>AQAGHYITKNGNDWQYDTNGELAKGLRQDSNGKLRYFDLTTGIQAKGQFVTIGQETYYFSKDHGDAQLLPMVTEGHYGTITLKQGQDTKTAWVYRDQNNTILKGLQNINGTLQFFDPYTGEQLKGGVAKY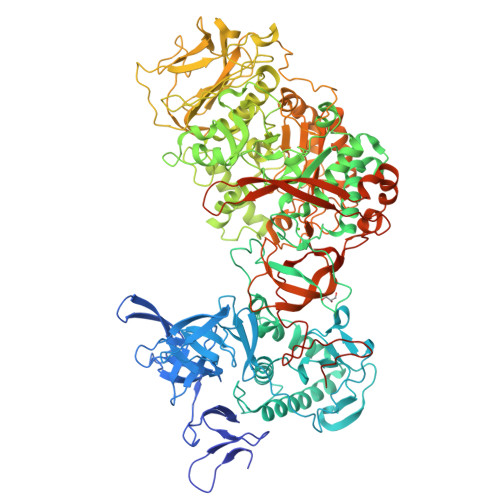DDKLFYFESGKGNLVSTVAGDYQDGHYISQDGQTRYADKQNQLVKGLVTVNGALQYFDNATGNQIKNQQVIVDGKTYYFDDKGNGEYLFTNTLDMSTNAFSTKNVAFNHDSSSFDHTVDGFLTADTWYRPKSILANGTTWRDSTDKDMRPLITVWWPNKNVQVNYLNFMKANGLLTTAAQYTLHSDQYDLNQAAQDVQVAIERRIASEHGTDWLQKLLFESQNNNPSFVKQQFIWNKDSEYHGGGDAWFQGGYLKYGNNPLTPTTNSDYRQPGNAFDFLLANDVDNSNPVVQAENLNWLHYLMNFGTITAGQDDANFDSIRIDAVDFIHNDTIQRTYDYLRDAYQVQQSEAKANQHISLVEAGLDAGTSTIHNDALIESNLREAATLSLTNEPGKNKPLTNMLQDVDGGTLITDHTQNSTENQATPNYSIIHAHDKGVQEKVGAAITDATGADWTNFTDEQLKAGLELFYKDQRATNKKYNSYNIPSIYALMLTNKDTVPRMYYGDMYQDDGQYMANKSIYYDALVSLMTARKSYVSGGQTMSVDNHGLLKSVRFGKDAMTANDLGTSATRTEGLGVIIGNDPKLQLNDSDKVTLDMGAAHKNQKYRAVILTTRDGLATFNSDQAPTAWTNDQGTLTFSNQEINGQDNTQIRGVANPQVSGYLAVWVPVGASDNQDARTAATTTENHDGKVLHSNAALDSNLIYEGFSNFQPKATTHDELTNVVIAKNADVFNNWGITSFEMAPQYRSSGDHTFLDSTIDNGYAFTDRYDLGFNTPTKYGTDGDLRATIQALHHANMQVMADVVDNQVYNLPGKEVVSATRAGVYGNDDATGFGTQLYVTNSVGGGQYQEKYAGQYLEALKAKYPDLFEGKAYDYWYKNYANDGSNPYYTLSHGDRESIPADVAIKQWSAKYMNGTNVLGNGMGYVLKDWHNGQYFKLDGDKSTLPQIKGELKLEGKPIPNPLLGLDSTRTGHHHHHH[4x]Muramidases (N-acetylmuramide glycanhydrolases), also known as lysozymes, cleave the bacterial cell wall peptidoglycan component at the β-1,4-glycosidic bond between N-acetylmuramic acid (NAM) and N-acetylglucosamine (NAG) in the carbohydrate backbone. The characterized enzymes from GH25 exhibit both β-1,4-N-acetyl- and β-1,4-N,6-O-diacetylmuramidase activities, cleaving the β-1,4-glycosidic bond between N-acetylmuramic acid (NAM) and N-acetylglucosamine (NAG) moieties in the carbohydrate backbone of bacterial peptidoglycan. The first half of the barrel, where the active site residues are located, is a classical barrel which is consistent with the idea that the initial ancient fold was a half-barrel which became an eight stranded barrel by gene duplication, with more sequence conservation in the half that contains the catalytic residue and less sequence (and as seen here structure) conservation in the other half which is responsible for binding specific targets. It is proposed that, as previously suggested for other GH25 muramidases, that Asp95 acts as an acid donating a proton to the glycosidic oxygen of the substrate, with the N-acetyl group of the substrate rather than a second protein carboxylate acting as the enzymatic nucleophile to stabilise the oxocarbenium ion-like transition state.

For TzMur, there were two independent protein molecules in the asymmetric unit, and the catalytic residues are Asp95 and Glu97. There are sulphate molecules from the crystallisation medium–one in subunit A and two in B. There are four glycerol molecules bound in each chain, introduced when adding the cryoprotectant. Three of these (numbered 301–303) lie in or close to the substrate-binding site, with the fourth one at the opposite side of the molecule. There is some residual difference density in the active site not good enough to be described as a ligand, the situation being complicated because the final crystals were obtained from the re-dissolved drops collected from other trays due to shortage of material. This density is described as water. Three of the GH25 structures have ligands bound, and, while we have not succeeded in obtaining a ligand complex, the structure of TzMur has four glycerol molecules from the cryoprotectant, three of which are in the ligand binding site. While most of the surrounding side chains from the binding sites superimpose very well, Tyr10 of TzMur and the corresponding aromatic residues from the other superimposed structures all have different conformations, indicating a high flexibility of the entrance to the binding site, which might facilitate optimal positioning of peptidoglycan for processing. TzMur, Zopfiella sp. t180-6 and Ascobolus stictoideus had Tm above 60°C at both pH 3 and 5. For both muramidases the optimum was around pH 4, independent of assay.

>[2x]AVPGFDISHYQPSVNYAGAYNSGARFVIIKATEGTTYTDPVFSTHYTGATKAGLIRGGYHFARPASSSGSAQADFFFKNGGGWSADGITLPGMLDMEYGSTSSCHGLSQTAMVNWISDFVNRYKTLSGRYPMIYTGYYWWVECTGNSNKFATTCPLVLARYSSSVGEIPGGWGYQTIWQFNDKYAYGGDSDSFNGSLDRLKALAKGT> GAAASGSEFMPVSVEELDATVRAFYEGRGEQQKAAQAALNQFKEDPDAWLMVDEILSRATYEQTKFLALQVLDNVIMTRWKVLPREQCQGIRNFVVQYILQCSSSEESLRTHRTLLNKLNLVLVSVLKQEWPHNWPTFINEIVSACHSSLSVCENNMIILRLLSEEVFDYSADQMTSTKTRNLKSTMCAEFSMIFQLCQEILNSATQPSLIKATLETLLRFCNWIPLGYIFETPLIDTLRTRFLEVPEFRNVTLQCLTEIGGLQTGGPGQPHTYDEQLIKMFTEVLTTISNIIPLQMDLKATYPNSNSRDQEFIQNLALFLTSFFTMHLPLIENLPNRDFLTHGHFYLIRISQIDDREIFKICLDYWLKLVQELYEEMQSLPLNDMSSMGLGMMSGGGAPNPALLEHYPLRKHKYKEVLSNLRVVMIEKMVRPEEVLIVENDEGEIVREFVKDTDSVQLYKTIRECLVYLTHLDVVDMEQI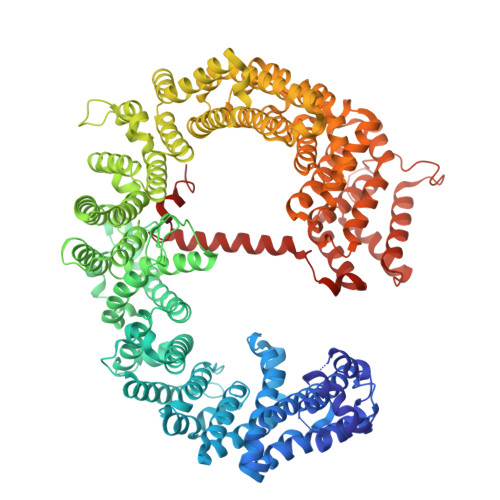MTEKLARQVDGSEWSWHNCNVLCWAIGSISMAMNEETEKRFLVTVIKDLLGLTEMKRGKDNKAVVASNIMYIVGQYPRFLKAHWKFLKTVVNKLFEFMHESHEGVQDMACDTFIKIAKQCRRHFVALQPSENEPFIEEIIRNIGKITCDLTPQQVHTFYEACGYMVSAQGNRNQQERLLAELMAIPNAAWDEIIKAATMNPGILHEPDTIKIIGNIMKTNVSACSSIGPYFFPQIGRLYNDMLQMYAATSQLISEAVARDGEIATKMPKVRGLRTIKKEILKLVETFVEKAEDLQAVRSQMIPGLLDSVLVDYNRNVPGARDAEVLKAMTVIITRLQGLMEDQVPAIMENVFECTLDMINKDFAEYPEHRVEFFNLLRAINLYCFPALLKLDNRQFKFVIDSCMWASKHDNRDVETAGLNMCLELINNIAEKTDVQTCNAFFNQFFIRILQDVFFVLTDTDHKAGFKTQSMLLMRLFYFVHPADGSAPKIQGPIYQPDQAQPGTGNREFLANFVGTLLQNAFANLTPLQITTFVKDCFELNTQYDKFRVVLRDFLISLREFAGDNAELYQVEKEQQEREARAADLERRSKVGGLLKPSELEDEEL> DKATIPSESPFAAAEVADGAIVVDIAKMKYETPELHVKVGDTVTWINREAMGHNVHFVAGVLGEAALKGPMMK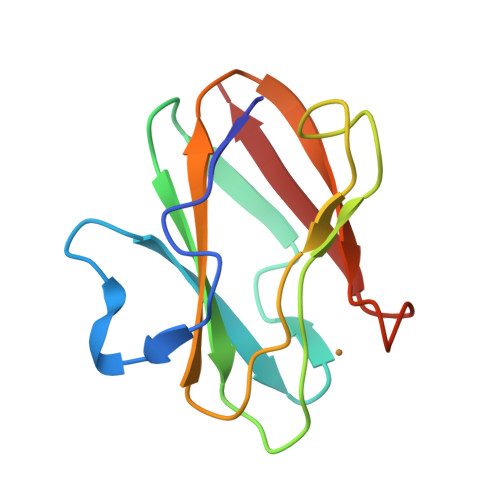KEQAYSLTFTEAGTYDYHCTPHPFMRGKVVVE>[2x]MSIEIRKLSIEDLETLIEVARESWKWTYAGIYSEEYIESWIREKYSKEKLLNEIVRSQSNLDILFLGAFADSTLIGFIELKIIANKAELLRLYLKPEYTHK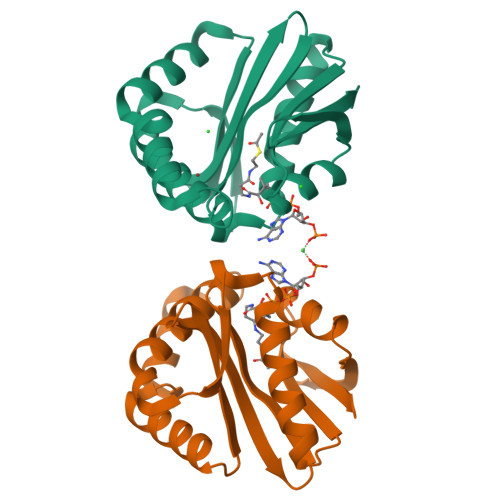KIGKTLLLEAEKIMKKKGILECRLYVHRQNSVGFSFYYKNGFKVEDTDGSDFIMEKKY The chicken avidin gene family consists of avidin and several avidin related genes (AVRs). In order to characterize the proteins encoded by the AVRs, avidin related proteins (AVRs) have recently been produced in insect cells using a baculovirus expression system and have been demonstrated to be functional biotin-binding proteins like chicken avidin. Interestingly, the biotin-binding affinities of AVRs have been reported to vary over a wide range of values, AVR4 being almost as efficient a biotin binder as avidin and AVR2 showing the lowest affinity for biotin. Each monomer in the homotetrameric protein has a β-barrel fold of eight β-strands with one end of the barrel adapted to bind D-biotin.

The X-ray structure of AVR2-b in complex with D-biotin was determined at 1.4 Å resolution. In AVR2, the O10B atom of D-biotin forms an additional hydrogen bond to the NE2 atom of Gln-97. Leucine in avidin (Leu-99) and AVR4 (Leu-97) is replaced by glutamine in AVR2 (Gln-97), and threonine in avidin (Thr-77) and AVR4 (Thr-75) is replaced by Ser-75 in AVR2. The side-chain atoms of Gln-97 of AVR2 not only interact with the valeryl segment of D-biotin, as in the case of the corresponding Leu in avidin and AVR4, but also with the carboxylate group of D-biotin (see above). The presence of the polar head group of Gln-97 in AVR2 also affects the type and conformation of the neighbouring residues, such as Ser-73, Leu-99 and Arg-112 as well as Ile-109 from another subunit. Ile-109 is found close to the biotin-binding site in AVR2, whereas all other proteins in avidin family have lysine at the equivalent position. In AVR2, Ile-109 resides close to Trp-108, which is known to be important for biotin binding, but the conformation of Trp-108 does not seem to be significantly affected by Ile-109. However, this substitution enlarges the binding cavity around bound biotin and hence contributes to the lower affinity of AVR2 for biotin. In AVR2, only valine (Val-113 in the AVRs) is conserved, while Met-96 and Ile-117 of avidin are respectively substituted by the hydrophilic residues Lys-94 and Asn-115 in AVR2. In the crystal structure of AVR2, the side chain of Lys-94 can exist in two alternate rotamers, which are hydrogen bonded either to the side-chain oxygen atom of Asn-115 or to the main-chain oxygen of Val-113, both from a neighbouring subunit. The conformation of the L3,4 loop of AVR2 was found to strongly resemble that of AVR4.

>[8x]QTVARKCSLTGEWDNDLGSIMTIGAVNDNGEFDGTYITAVADNPGNITLSPLLGIQHKRASQPTFGFTVHWNFSESTSVFVGQCFVDRSGKEVLKTKWLQRLAVDDISDDWIATRVGNNDFTRQHTVEE> ADYQVYAWGINDPTEGERTVIKDPWDSVASEFTWISDGSTNYTTSRGNNGIAQSNPSGGPSY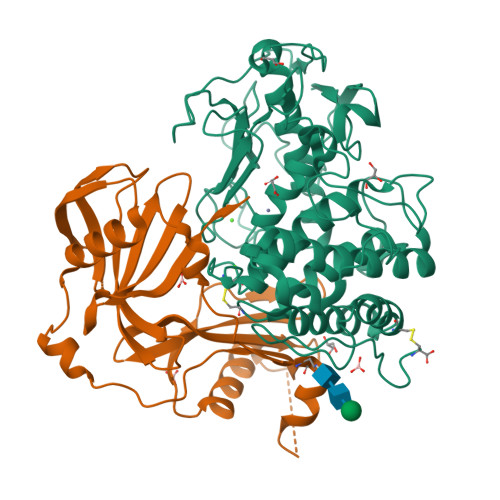LNNYRPSSSSLSFKYPYSVSSSPPSSYIDASIIQLFYTANIYHDLLYTLGFTEKAGNFEYNTNGQGGLGNDYVILNAQDGSGTNNANFATPPDGQPGRMRMYVWTESTPYRDGSFEAGIVIHEYTHGLSNRLTGGPANSNCLNALESGGMGEGWSDFMATAIRLKPGDKRSTDYTMGEWASNRAGGIRQYPYSTSLSTNPLTYTSVNSLNAVHAIGTVWASMLYEVLWNLIDKHGKNDAPKPTLRDGVPTDGKYLAMKLVMDGMALQPCNPNFVQARDAILDADTALTGGENQCEIWTAFAKRGLGAGAKYSSRNRVGSTEVPSGVC;> TVDLNAFRLKSLAKYVNATETVIEAPSSFAPFKPQSYVEVATQHVKMIAPDATFRVVDDHYVGDNGVAHVHFRQTANGLDIDNADFNVNVGKDGKVFSYGNSFYTGQIPSSAALTKRDFSDPVTALKGTTNTLQLPITVDSASSESTEEKESYVFKGVSGTVSDPKAKLVYFVKDDGTLALAWRVETDIDSNWLLTYIDAKSGEEIHGVVDYVAE>[9x]FTLVELIVVIIIIAIIAAVAIPAITSFQDNARKSRIQSEHRELVSAIQSYIGAQDDPTNPSEITLAKLAPYMSKNAKNE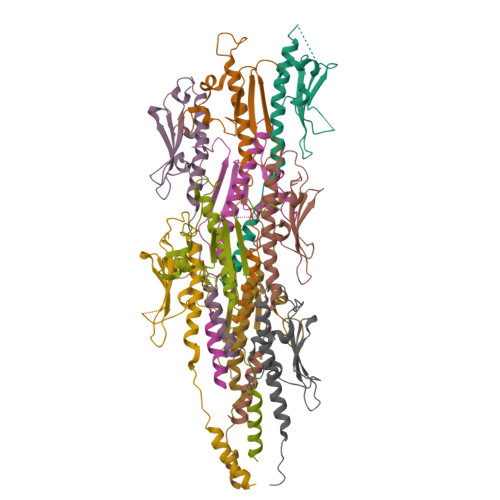DGIVNSLAKDKSGNSSTSAPGSAHQIDTTNHKLISTFTPSNGGQATVLTYDWSANGVNSN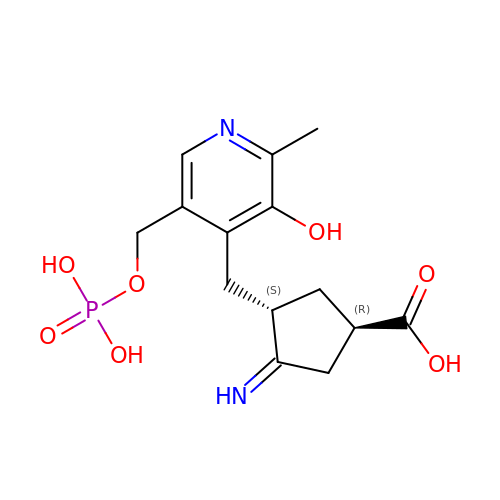(1R,3S,4Z)-3-({3-hydroxy-2-methyl-5-[(phosphonooxy)methyl]pyridin-4-yl}methyl)-4-iminocyclopentane-1-carboxylic acid | C14 H19 N2 O7 P | CTOWFYUCLIAQOJ-XPIHRMQRSA-N>MASDVTVNVSAEKQVIRGFGGMNHPAWAGDLTAAQRETAFGNGQNQLGFSILRIHVDENRNNWYKEVETAKSAVKHGAIVFASPWNPPSDMVETFNRNGDTSAKRLKYNKYAAYAQHLNDFVTFMKNNGVNLYAISVQNEPDYAHEWTWWTPQEILRFMRENAGSINARVIAPESFQYLKNLSDPILNDPQALANMDILGTHLYGTQVSQFPYPLFKQKGAGKDLWMTEVYYPNSDTNSADRWPEALDVSQHIHNAMVEGDFQAYVWWYIRRSYGPMKEDGTISKRGYNMAHFSKFVRPGYVRIDATKNPNANVYVSAYKGDNKVVIVAINKSN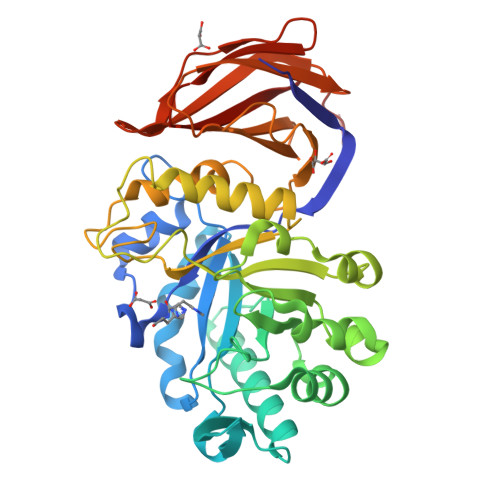TGVNQNFVLQNGSASNVSRWITSSSSNLQPGTNLTVSGNHFWAHLPAQSVTTFVVNRLEHHHHHHHH[4x]>[2x]IPEYVDWRQKGAVTPVKNQGSCGSC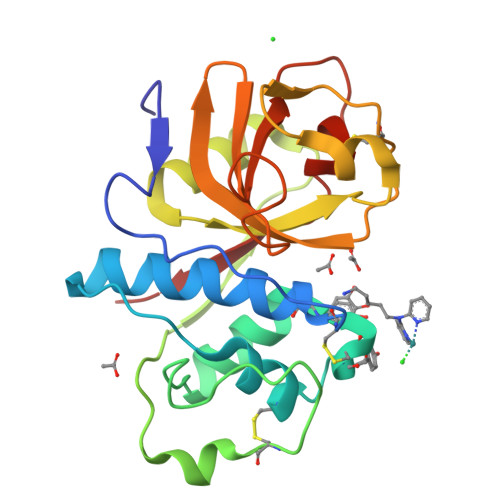WAFSAVVTIEGIIKIRTGNLNEYSEQELLDCDRRSYGCNGGYPWSALQLVAQYGIHYRNTYPYEGVQRYCRSREKGPYAAKTDGVRQVQPYNEGALLYSIANQPVSVVLEAAGKDFQLYRGGIFVGPCGNKVDHAVAAVGYGPNYILIKNSWGTGWGENGYIRIKRGTGNSYGVCGLYTSSFYPVKN> GSAEEWYFGKI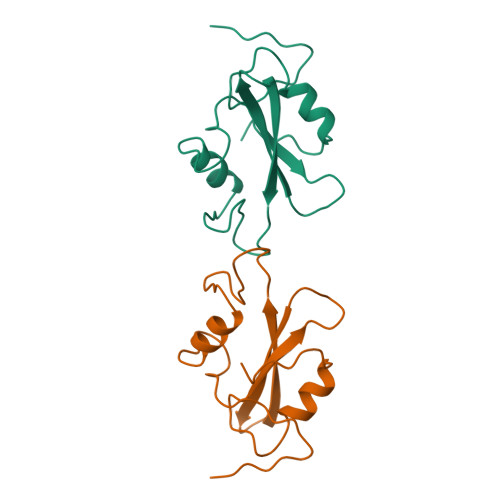TRRESESLLLNPENPRGTFLVRESETTKGAYCLSVSDFDNAKGLNVKHYKIRKLDSGGFYITSRTQFSSLQQLVAYYSKHADGLCHRLTNVCPTSKEFIVTD>GGSGNEPTQEKHFMVYYRAWRDKTMQGVNTTLPDENWLTMHDIPYGIDIVNVFSYVPKGQEALAQPFYDTLKNEYAPALHARGVRLVRGIDYSELLKVPYAGTTPTEAEFDAYAKELLTKFVDDLGIDGLDIDMETRPSEKDIVLSNGVIRALSKYIGPKSGTDRPFLYDTNAEYLPPLQDVSDCFDFLAYQQYGSDDKRTQRALNNLSPVLNGERFVPGLTFPEEQDRNRWYDTKEPYMESNMYKVARYSYENNLGGMFLYALDRDGRTYNEDDLNQIKPSNLLWTKTAIAESKGVSLAEMKAAAQHYLKRISYANTDLEAQNKAAETVTQAT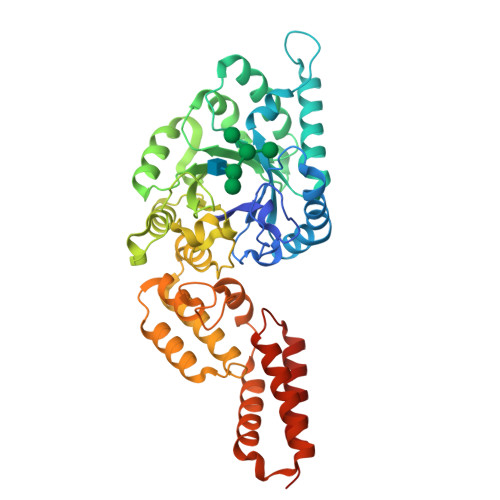TLYDVNKAILGGDYGQGLSNTYDAELEKGLLAIDLTTLYRALDQAVAAIEKAESYTPETIQALQTTKESVATELAGKTYTAAQVTTWQTEVQTALDNLKEK[2x]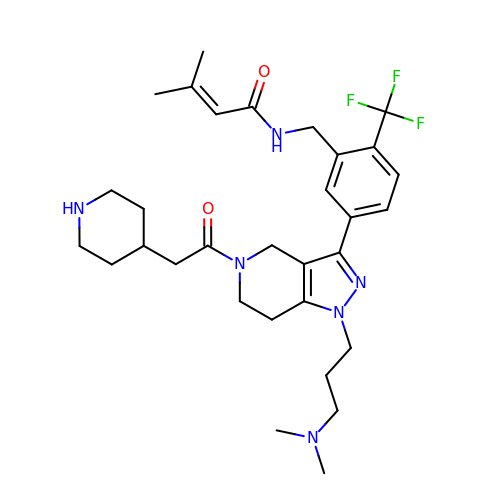N-{[5-{1-[3-(dimethylamino)propyl]-5-[(piperidin-4-yl)acetyl]-4,5,6,7-tetrahydro-1H-pyrazolo[4,3-c]pyridin-3-yl}-2-(trifluoromethyl)phenyl]methyl}-3-methylbut-2-enamide | C31 H43 F3 N6 O2 | YYKUWQZWTBVESL-UHFFFAOYSA-N Microsomal glutathione S-transferase 2 (MGST2) is a member of a family of integral membrane proteins denoted MAPEG (Membrane Associated Proteins in Eicosanoid and Glutathione metabolism), which encompasses several important targets for development of anti-inflammatory and anti-cancer drugs interfering with prostaglandin and leukotriene biosynthesis. In non-hematopoietic cells, MGST2 catalyzes leukotriene C4 (LTC4) synthesis via conjugation of glutathione (GSH) and LTA4, a transient epoxide intermediate derived from 5-lipoxygenase metabolism of arachidonic acid. Previous studies of MGST2 have revealed that only one out of three active sites is used at a time, an intriguing catalytic behavior also observed for MGST1 and microsomal prostaglandin E synthase-1 (mPGES-1) both of which are strongly implicated in human pathophysiology. The overall structure is a homo-trimer, with each monomer containing 4 trans-membrane α-helices (αH1–αH4), forming three potential active sites at their interfaces.

The structure of apo-MGST2 (with two homo-trimers in the asymmetric unit) shows structural heterogeneity, while the structure of holo-MGST2, which contains GSH at only two of the three possible active sites appears more rigid. In the holo structure, only one of the GSH molecules is observed in full occupancy, with the other refined to 72%. The binding conformation of GSH as well as those of associated interactions with active site residues differs markedly between these two sites, suggesting that only the GSH at full occupancy is bound productively. The GSH at full occupancy observed in the holo complex adopts a “crescent”-shaped binding mode, similar to what has been reported for LTC4 synthase10,11 and mPGES-112, while contrasting to the extended conformation described for MGST1. In comparison, the GSH at partial occupancy displays several distinct features. This GSH has an opposite head to tail orientation with its γ-glutamyl amino group hydrogen bonded to Tyr97 instead of Glu58 as for the GSH at full occupancy. Furthermore, the salt bridge between Arg51 and the glycyl carboxylate of GSH is lost at the partially occupied site, which contributes to its inefficient binding. In the holo–GSH complex, however, this region adopts a loop conformation with relatively high B-factor within the unoccupied active site. This transition from 310 helix to loop makes the essential Arg104 more flexible, which is reflected in poor electron density compared with GSH-bound sites. In contrast, in the holo state, the productively bound GSH interacts tightly within the active site, which globally rigidifies MGST2.

>MHHHHHHAGNSILLAAVSILSACQQSYFALQVGKARLKYKVTPPAVTGSPEFERVFRAQQNCVEFYPIFIITLWMAGWYFNQVFATCLGLVYIYGRHLYFWGYSEAAKKRITGFRLSLGILALLTLLGALGIANSFLDEYLDLNIAKKLRRQF[3x]>AVELNTFQNIVDAIAEGKRITFVINLKKCTSEMPLNSAIVSVTPNAVMVIGDSRVTASDRHFTLDDPLARGTPMFDYSKFNLDSEGDASIKTTVLNASSYERLGSY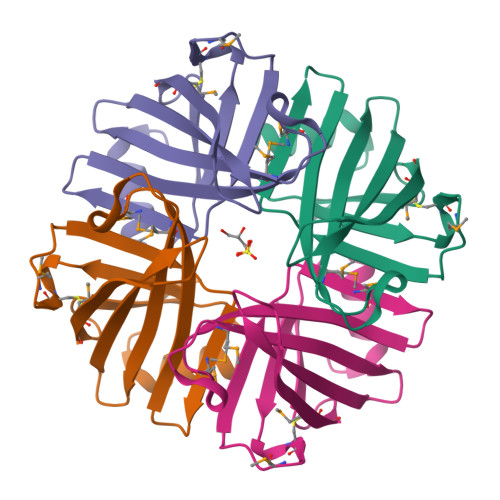QMNCKLGDGFKVFG[4x]>CGTACG[2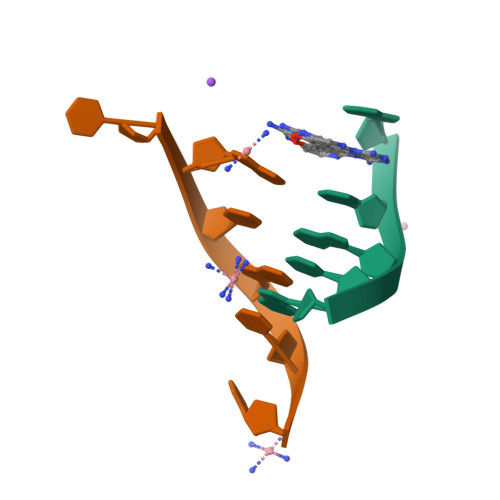x]> GPVEDAITAAIGRVADTVGTGPTNSEAIPALTAAETGHTSQVVPGDTMQTRHVKNYHSRSESTIENFLCRSACVYFTEYENSGAK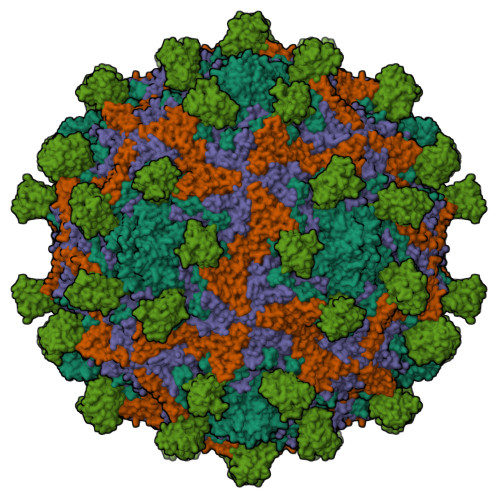RYAEWVLTPRQAAQLRRKLEFFTYVRFDLELTFVITSTQQPSTTQNQDAQILTHQIMYVPPGGPVPDKVDSYVWQTSTNPSVFWTEGNAPPRMSIPFLSIGNAYSNFYDGWSEFSRNGVYGINTLNNMGTLYARHVNAGSTGPIKSTIRIYFKPKHVKAWIPRPPRLCQYEKAKNVNFQPSGVTTTRQSITTMTNTGAF;> SPTVEECGYSDRARSITLGNSTITTQECANVVVGYGVWPDYLKDSEATAEDQPTQPDVATCRFYTLDSVQWQKTSPGWWWKLPDALSNLGLFGQNMQYHYLGRTGYTVHVQCNASKFHQGCLLVVCVPEAEMGCATLDNTPSSAELLGGDSAKEFADKPVASGSNKLVQRVVYNAGMGVGVGNLTIFPHQWINLRTNNSATIVMPYTNSVPMDNMFRHNNVTLMVIPFVPLDYCPGSTTYVPITVTIAPMCAEYNGLRLAGHQ;> GLPTMNTPGSCQFLTSDDFQSPSAMPQYDVTPEMRIPGEVKNLMEIAEVDSVVPVQNVGEKVNSMEAYQIPVRSNEGSGTQVFGFPLQPGYSSVFSRTLLGEILNYYTHWSGSIKLTFMFCGSAMATGKFLLAYSPPGAGAPTKRVDAMLGTHVVWDVGLQSSCVLCIPWISQTHYRYVTSDEYTAGGFITCWYQTNIVVPADAQSSCYIMCFVSACNDFSVRLLKDTPFISQQNFFQ;> MGAQVSTQKTGAHETGLNASGNSIIHYTNINYYKDAASNSANRQDFTQDPGKFTEPVKDIMIKSLPALN;> MSITTPEEMIEKAKGETAYLPCKFTLSPEDQGPLDIEWLISPADNQKVDQVIILYSGDKIYDDYYPDLKGRVHFTSNDLKSGDASINVTNLQLSDIGTYQCKVKKAPGVANKKIHLVVLVKPSGARCYVDGSEEIGSDFKIKCEPKEGSLPLQYEWQKLSDSQKMPTSWLAEMTSSVISVKNASSEYSGTYSCTVRNRVGSDQCLLRLNVVPPSNKALEHHHHHH>GSDGDALLKPCKLGDMQCLSSATEQFLEKTSKGIPQYDIWPIDPLVVTSLDVIAPSDAGIVIRFKNLNITGLKNQQISDFQMDTKAKTVLLKTKADLHIVGDIVIELTEQSKSFTGLYTADTNVIGAVRYGYNLKNDDNGVQHFEVQPETFTCESIGEPKITLSSDLSSALEKDSGNNSLEPDMEPLKTLRQAAICKIAEACYISV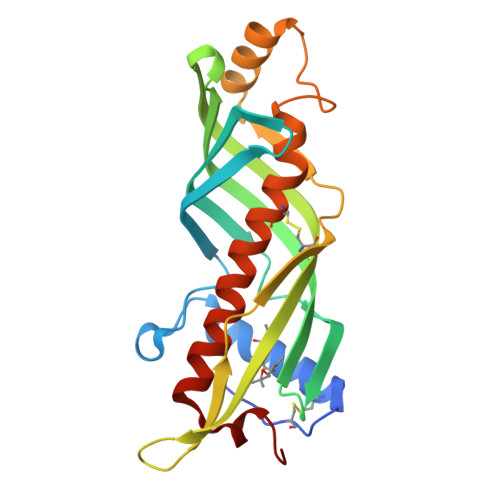VHNIRASAKILPASSFFENLN[2x]>[16x]GSRPTD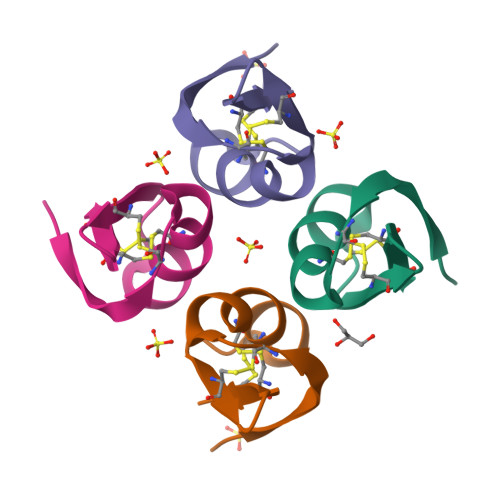IKCSASYQCFPVCKSRFGKTNGRCVNGLCDCF>[2x]GPMEIIRSNFKINLHKVYQAIEEADFFAIDGEFSGISDGPSVTALTSGFDTPEERYQKLKKHSMDFLLFQFGLCAFKYDHTDSKHVTKSFNFYVFPKPFSRSSPDVKFVCQSSSIDFLASQGFDFNKVFCSGIPYLNQEEERQLREQFDEKRSQANGAGALAKCPVTIPEDQKKFIDQVIEKIEDFLQSEEKRSLELDPCTGFQRKLIYQTLSWKYPKGIHVETLETDKKERHIVISKVDEEERKRREQEKYTKEQEELNDAVGFSRVIHAIANSGKLVVGHNML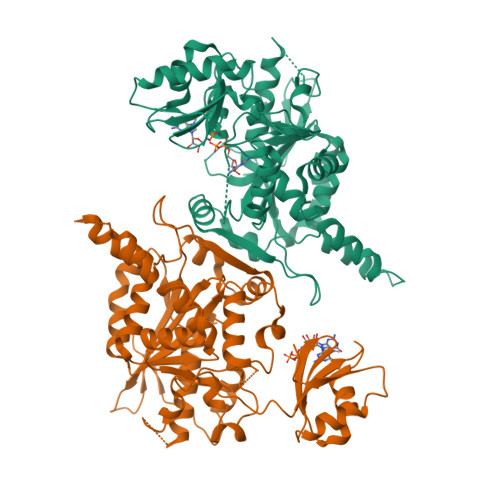LDVMHTIHQFYCPLPADLNEFKEMAICVFPRLLDTKLMASTQPFKDIINNTSLAELEKRLKETPFDPPKVESAEGFPSYDTASEQLHEAGYDAYITGLCFISMANYLGSLLSPPKMCVSARSKLIEPFFNKLFLMRVMDIPYLNLEGPDLQPKRDHVLHVTFPKEWKTSDLYQLFSAFGNIQISWIDDTSAFVSLSQPEQVQIAVNTSKYAESYRIQTYAEY> MLEAKFEEASLFKRIIDGFKDCVQLVNFQCKEDGIIAQAVDDSRVLLVSLEIGVEAFQEYRCDHPVTLGMDLTSLSKILRRGNNTDTLTLIADNTPDSIILLFEDTKKDRIAEYSLKLMDIDADFLKIEELQYDSTLSLPSSEFSKIVRDLSQLSDSINIMITKETIKFVADGDIGSGSVIIKPFV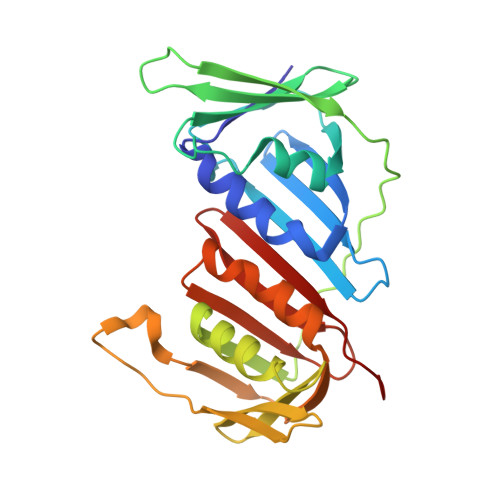DMEHPETSIKLEMDQPVDLTFGAKYLLDIIKGSSLSDRVGIRLSSEAPALFQFDLKSGFLQFFLAPKFND> SLLVPANPYHTAEIPDWLQVYARAPVKYDHILKWELFQLADLDTYQGMLKLLFMKELEQ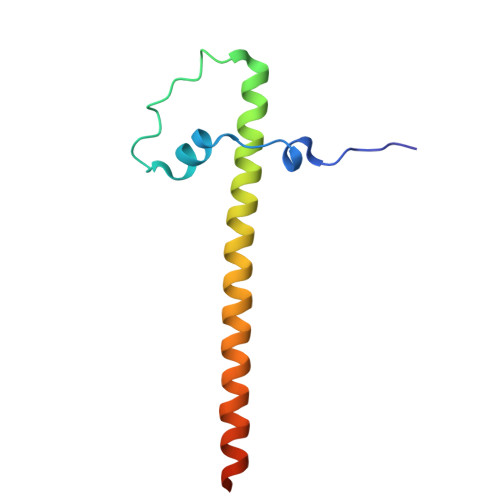IVKMYEAYRQALLTELENRKQRQQWYAQQHGKNF>MKFMVEVRIRLKKGMLNPEAATIERALALLGYEVEDTD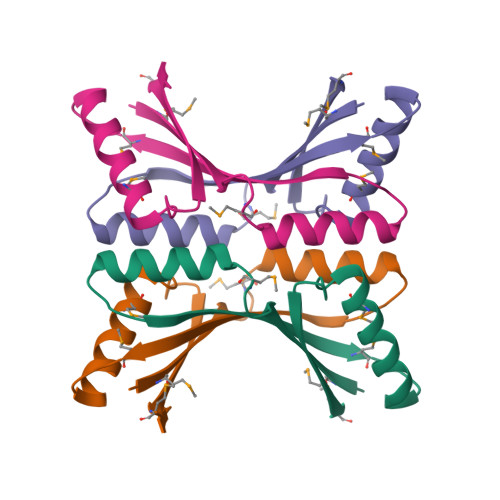TTDVITFTMDEDSLEAVEREVEDMCQRLLCNPVIHDYDVSINEMSSH[2x]We previously identified a circular bacteriocin plantacyclin B21AG from Lactiplantibacillus plantarum B21 (previously known as Lactobacillus plantarum). This family II circular bacteriocin has antimicrobial activity against foodborne pathogens including Listeria monocytogenes and Clostridium perfringens and other closely related Lactobacillus species. Of these, circular bacteriocins (class I) have gained attention due to their unique characteristics of high thermal and pH stability, as well as resistance to degradation by many proteolytic enzymes. The covalently linked N- and C-termini form a structurally distinct cyclic peptide backbone.

In the present study, we report the crystal structure of plantacyclin B21AG. A crystal from these conditions diffracted to 1.8 Å resolution and belonged to the space group C2221. The crystal structure diffraction data were phased by molecular replacement using a theoretical α-helix (8 residues long polyalanine) as a search model. There are two independent molecules of plantacyclin B21AG in the asymmetric unit. The structures of these two molecules (Chain A and Chain B) are similar to each other, with a Cα backbone root-mean-square deviation, RMSD of 0.56 Å across 58 Cα atoms. The four α-helices in the crystal structure are connected by loops of 1 to 6 residues and enclose a hydrophobic core in a tightly folded globular arrangement. Helix α1 and helix α4 are linked covalently between Ile1 and Ala58 in the middle of helix α4, creating a circular backbone. The second, third and fourth α-helices are predominantly hydrophobic, with the linked amino acids at the N- and C-termini in helix α4 buried in the core of the structure. In contrast, helix α1 is amphipathic, with hydrophilic residues (Thr14, Gln18, Ser25 and Ser26) exposed at the surface of the protein. The protein has an overall net charge of + 3 at physiological pH, with four cationic residues located in helix α1 (Lys15 and Lys19), helix α4 (Arg6) and the loop connecting α1/α4 (His11), and one anionic residue located in helix α1 (Asp22).

>[2x]IVWIARQFGVHLTTKLTQKALDLLSSGASLGTVAAVILGVTLPGWAVAAAGALGGTAA>[12x]MFEIKK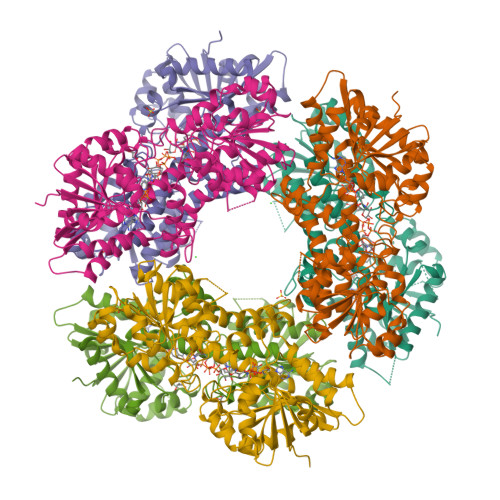ICCIGAGYVGGPTCSVIAHMCPEIRVTVVDVNESRINAWNSPTLPIYEPGLKEVVESCRGKNLFFSTNIDDAIKEADLVFISVNTPTKTYGMGKGRALDLKYIEACARRIVQNSNGYKIVTEKSTVPVRAAESIRRIFDANTKPNLNLQVLSNPEFLAEGTAIKDLKNPDRVLIGGDETPEGQRAVQALCAVYEHWVPREKILTTNTWSSELSKLAANAFLAQRISSINSISALCEATGADVEEVATAIGMDQRIGNKFLKASVGFGGSCFQKDVLNLVYLCEALNLPEVARYWQQVIDMNDYQRRRFASRIIDSLFNTVTDKKIAILGFAFKKDTGDTRESSSIYISKYLMDEGAHLHIYDPKVPREQIVVDLSHPGVSEDDQVSRLVTISKDPYEACDGAHAVVICTEWDMFKELDYERIHKKMLKPAFIFDGRRVLDGLHNELQTIGFQIETIGKKVSSKRIPYAPSGEIPKFSLQDPPNKKPKV>MGDRSDHAKKLKTFLENLRRHLDRLDKHIKQLRDILSENPEDE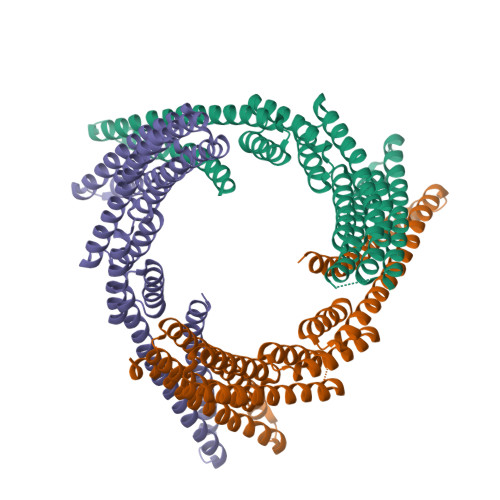RVKDVIDLSERSVRIVKTVIKIFEDSVRKLLKQINKEAEELAKSPDPEDLKRAVELAEAVVRADPGSNLSKKALEIILRAAAELAKLPDPDALAAAARAASKVQQEQPGSNLAKAAQEIMRQASRAAEEAARRAKETLEKAEKDGDPETALKAVETVVKVARALNQIATMAGSEEAQERAARVASEAARLAERVLELAEKQGDPEVARRARELQEKVLDILLDILEQILQTATKIIDDANKLLEKLRRSERKDPKVVETYVELLKRHERLVKQLLEIAKAHAEAVEGGSLEHHHHHH[6x]>LTPDQQTLLHFIMDSYNKQRMPQEITNKILKEEFSAEENFLILTEMATNHVQVLVEFTKKLPGFQTLDHEDQIALLKGSAVEAMFLRSAEIFNKKLPSGHSDLLEERIRNSGISDEYITPMFSFYKSIGELKMTQEEYALLTAIVILSPDRQYIKDREAVEKLQE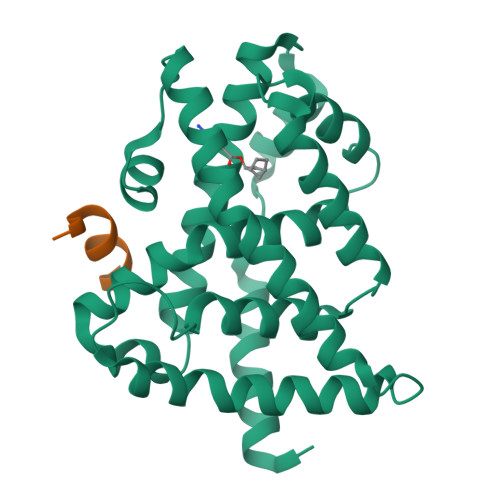PLLDVLQKLCKIHQPENPQHFACLLGRLTELRTFNHHHAEMLMSWRVNDHKFTPLLCEIWDV[2x];>[2x]ENLLLRYLLDK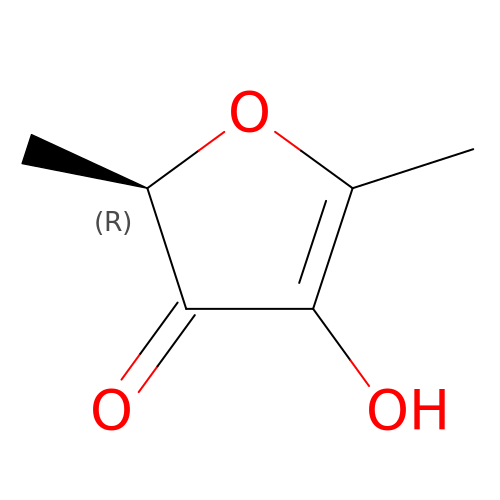(2R)-4-hydroxy-2,5-dimethylfuran-3(2H)-one | C6 H8 O3 | INAXVXBDKKUCGI-GSVOUGTGSA-N>AAPSFDCGKPQVEPKKCPGRVVGGCVAHPHSWPWQVSLRTRFGMHFCGGTLISPEWVLTAAHCLEKSPRPSSYKVILGAHQEVNLEPHVQEIEVSRLFLEPTRKDIALLKLSSPAVITDKVIPACLPSPNYVVADRTECFITGWGETQGTFGAGLLKEAQLPVIENKVCNRYEFLNGRVQSTELCAGHLAGGTDSCQGDAGGPLVCFEKDKYILQGVTSWGLGCARPNKPGVYVRVSRFVTWIEGVMRNN[2x];>[2x]SVNNSQLVVSVAGTVEGTNQDISLKFFEIDLTSRPAHGGKTEQGLSPKSKPFATDSGAMPHKLEKADLLKAIQEQLIANVHSNDDYFEVIDFASDATITDRNGKVYFADKDGSVTLPTQPVQEFLLSGHVRVRPYKEKPIQNQAKSVDVEYTVQFTPLNPDDDFRPGLKDTKL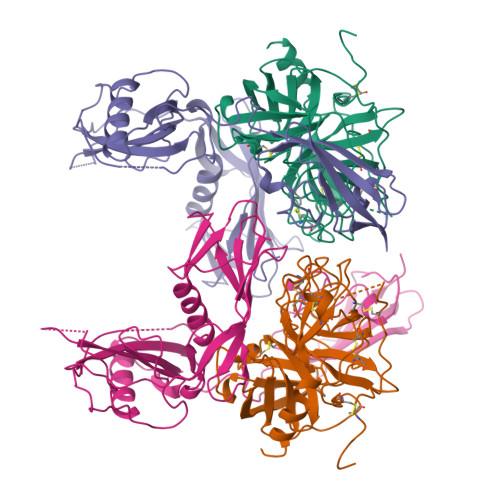LKTLAIGDTITSQELLAQAQSILNKTHPGYTIYERDSSIVTHDNDIFRTILPMDQEFTYHVKNREQAYEINKKSGLNEEINNTDLISEKYYVLKKGEKPYDPFDRSHLKLFTIKYVDVNTNELLKSEQLLTASERNLDFRDLYDPRDKAKLLYNNLDAFGIMDYTLTGKVEDNHDDTNRIITVYMGKRP(cyclohexylamino)(oxo)acetic acid | C8 H13 N O3 | 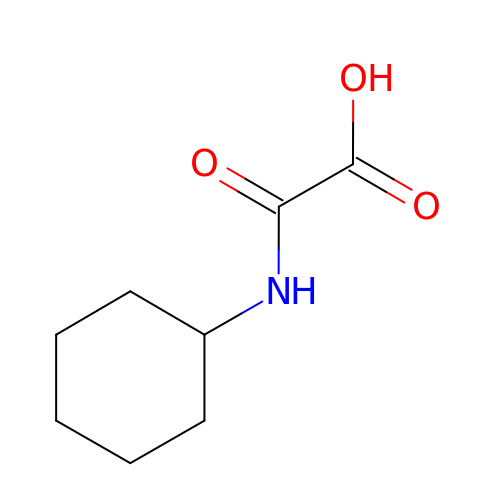JXKXKOUBASQQOF-UHFFFAOYSA-N(3~{S})-1-ethanoyl-3-(4-methylphenyl)piperidine-3-carboxylic acid | C15 H19 N O3 | 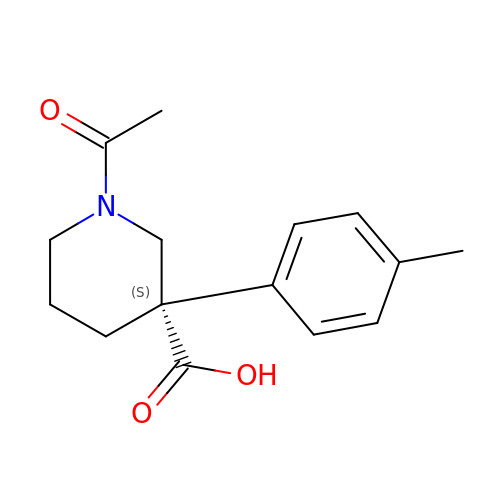FZGIXDHLUQHJKF-OAHLLOKOSA-N>MGSSEQLHEPAELLSEETKNMHRALVTLIEELEAVDWYQQRADACSEPGLHDVLIHNKNEEVEHAMMTLEWIRRRSPVFDAHMRTYLFTERPILELEE[10x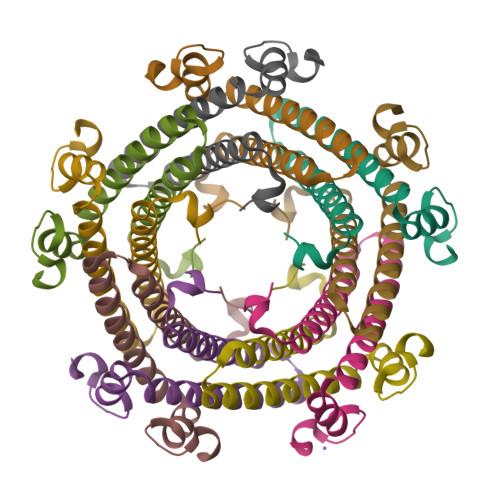]> MDYKDDDDKSPGGSMELLCCEGTRHAPRAGPDPRLLGDQRVLQSLLRLEERYVPRASYFQCVQREIKPHMRKMLAYWMLEVCEEQRCEEEVFPLAMNYLDRYLSCVPTRKAQLQLLGAVCMLLASKLRETTPLTIEKLCIYTDHAVSPRQLRDWEVLVLGKLKWDLAAVIAHDFLAFILHRLSLPRDRQALVKKHAQTFLALCATDYTFAMYPPSMIATGSIGAAVQGLGACSMSGDELTELLAGITGT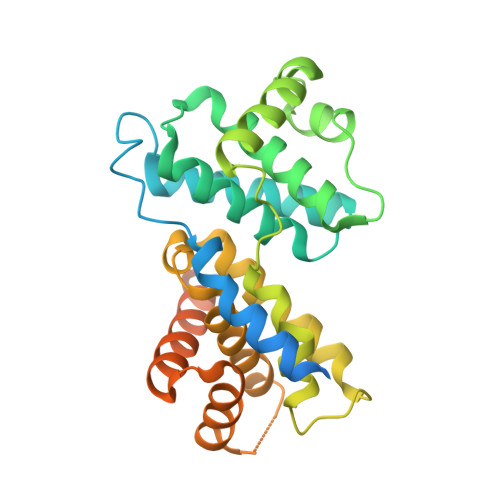EVDCLRACQEQIEAALRESLREAAQTSSSPAPKAPRGSSSQGPSQTSTPTDVTAIHL>GSGSMKDYDELLKYYELHETIGTGGFAKVKLACHILTGEMVAIKIMDKNTLGSDLPRIKTEIEALKNLRHQHICQLYHVLETANKIFMVLEYCPGGELFDYIISQDRLSEEETRVVFRQIVSAVAYVHSQGYAHRDLKPENLLFDEYHKLKLIDFGLCAKPKGNKDYHLQTCCGSLAYAAPELIQGKSYLGSEADVWSMGILLYVLMCGFLPFDDDNVMALYKKIMRGKYDVPKWLSPSSILLLQQMLQVDPKKRISMKNLLNHPWIM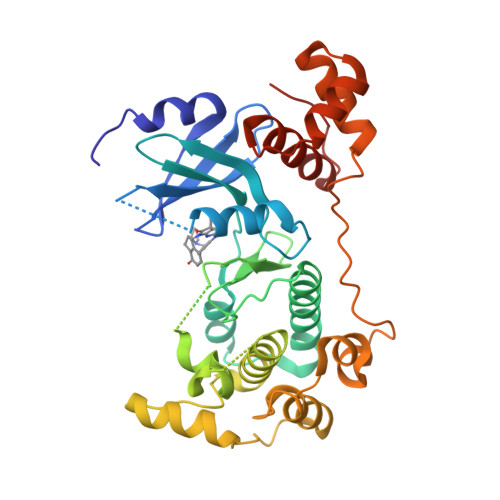QDYNYPVEWQSKNPFIHLDDDCVTELSVHHRNNRQTMEDLISLWQYDHLTATYLLLLAKKARGKPVRLRLSSFSCG[2x]>NGEEHEQ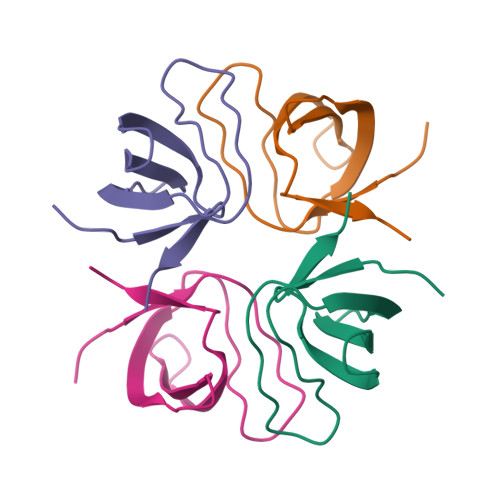THRAIFRFVPRHEDELELEVDDPLLVELQAEDYWYEAYNMRTGARGVFPAYYAIEVTKEPEHMA[4x]> MGSSHHHHHHSQDPMSRQANRGTESKKMSSELFTLTYGALVTQLCKDYENDEDVNKQLDKMGFNIGVRLIEDFLARSNVGRAHDFRETADVIAKVAFKMYLGITPSITNWSPAGDEFSLILENNPLVDFVELPDNH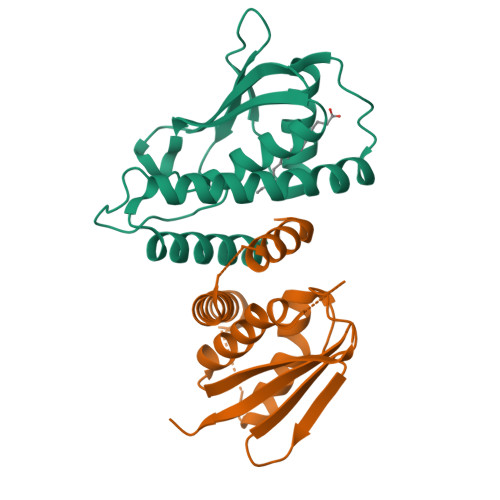SSLIYSNLLCGVLRGALEMVQMAVEAKFVQDTLKGDGVTEIRMRFIRRIEDNLPAGEE;> MADEALFLLLHNEMVSGVYKSAEQGEVENGRCITKLENMGFRVGQGLIERFTKDTARFKDELDIMKFICKDFWTTVFKKQIDNLRTNHQGIYVLQDNKFRLLTQMSAGKQYLEHASKYLAFTCGLIRGGLSNLGIKSIVTAEVSSMPACKFQVMIQKL> KPEPTDEEWELIKTVTEAHVATNAQGSHWKQKRKFLPEDIGQAPIVNAPEGGKVDLEAFSHFTKIITPAITRVVDFAKKLPMFCELPCEDQIILLKGCCMEIMSLRAAVRYDPESETLTLNGEMAVTRGQLKNGGLGVVSDAIFDLGMSLSSFNLDDTEVALLQAVLLMSSDRPGLACVERIEKYQDSFLLAFEHYINYRKHHVTHFWPKLLMKVTDLRMIGACLASRFLHMKVECPTELFPPLFLEV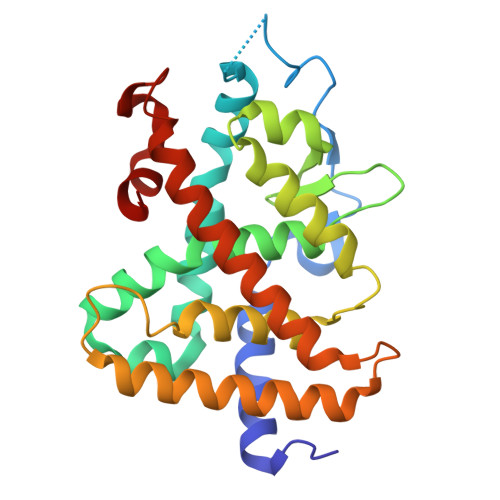F>[2x]TVFRQENVDDYYDTGEELGSGQFAVVKKCREKSTGLQYAAKFIKKRRTKSSRRGVSREDIEREVSILKEIQHPNVITLHEVYENKTDVILILELVAGGELFDFLAEKESLTEEEATEFLKQILNGVYYLHSLQIAHFDLKPENIMLLDRNVPKPRIKIIDFGLAHKIDFGNEFKNIFGTPEFVAPEIVNYEPLGLEADMWSIGVITYILLSGASPFLGDTKQETLANVSAVN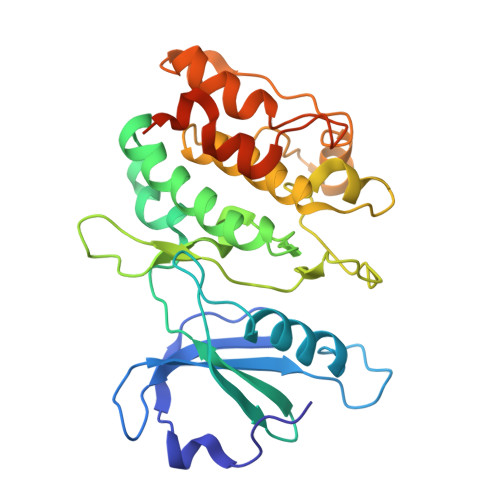YEFEDEYFSNTSALAKDFIRRLLVKDPKKRMTIQDSLQHPWIKPKDTQQALSSAWSHPQFEK Nucleoside monophosphate (NMP) kinases are ubiquitous enzymes in the biosynthesis and regeneration of ribonucleoside and deoxyribonucleoside triphosphates. Prokaryotic UMPKs have no sequence similarity to other known NMP kinases but have significant sequence and structural similarity to amino acid kinases including aspartokinases and glutamate kinases. Generally, the activity of bacterial UMPKs is stimulated by GTP, whereas that of archaeal UMPKs is not. One hexamer comprises chains A, B and C, whereas the other two comprise chains D, E, F, G, H and I. The hexamer has the architecture of a trimer of dimers, which is common to other bacterial UMPKs.

We determined the crystal structure of UMP kinase of an extreme thermophile Thermus thermophilus HB8 in ADP-UDP–bound form at 2.6-Å resolution. The structure of the ADP-UDP complex is the first structure of bacterial UMP kinase with a phosphoryl group donor and an acceptor. The crystal belongs to space group I222 and contains nine ttUMPK molecules (chains A–I) per asymmetric unit. The subunit of ttUMPK has an α/β-fold with a eight-stranded β-sheet surrounded by eight α-helices and one 310 helix. In the determined structure, ADP is located between the αF-αG and β4-β5 loops, as is common among archaeal UMPK structures. The β-phosphate moiety interacts with the side chains of Lys9 (3.0 Å), Ser11 (2.9 Å) and Lys157 (2.7 Å), the main-chain amide of Asn158 (3.0Å) and a magnesium ion (2.5 Å). UDP is located among the β1-αA, β2-αC and β4-αE loops, as is common among other bacterial UMPK structures. The magnesium ion is coordinated by four oxygen atoms from the α- and β-phosphates of ADP as well as the β-phosphate of UDP and one water molecule (2.9 Å), and it may be coordinated by the side chain of Ser136 (3.4 Å). Furthermore, in the UDP-ADP form of ttUMPK, the corresponding loop is closer to the active site than the UDP form of ecUMPK (magenta). The Cα atom of Lys170 of ttUMPK, corresponding to Lys177 of ecUMPK, shifts 4.0 Å compared with the UDP-bound ecUMPK. This motion enables Asp167, Arg169 and Tyr164 to interact with the bound ADP.

>[9x]MKYKRVLLKLSGEFLTRNGFGIEPEATQALAREIKAAYDTGVQLAIVIGAGNLWRGARQGVGMDRATADYIGMLATIMNALALQDALESLGVPTRVQTALTITQVAEPYIRRRALRHLEKERIVIFGGGTGNPFFSTDTAAALRALEVGAEVVLMAKNKVDGVYSDDPRKNPEAVRFDELTYLEVLNRGLQVMDTTAITLCMEAGLPIVVFDIFKPGALVGIIQGEKVGTLIH> SEKKNYSALFENLQNRSNPEKLQEITTKFFSDNPDVKYNDVLKYITLAMNGVSPEYTNKSREAGEKVKLHLQDILLDVEYQYQGSVM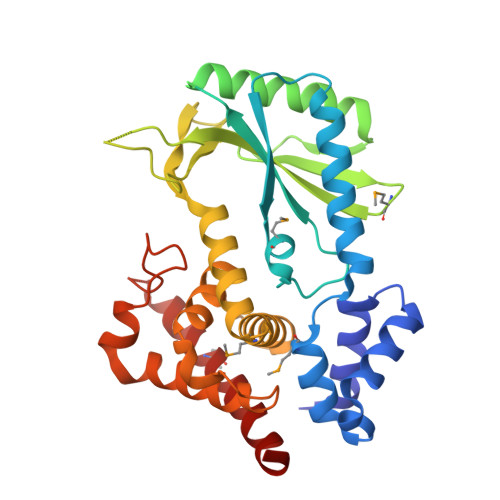TNTHIKGYSDIDLLVISDKFYTLDERNIIENLEVNKFSLSQEKIQKLQQELLGKKYHSATNDLKNNRLLSEQKLSSVYEICDITHPKAIKITNKSMGRDVDIVIANWYDDAQSVINNRQIEYRGIQIYNKRSNTIENRDFPFLSIQRINKRSSETKGRLKKMIRFLKNLKADSDEKIELSSFDINAICYNIEKNKYLHSNKYQLVPILYEQLNELVSNSNKINSLKSVDGHEYIFSRNNIDKKESLKMLLQEVKIIYSNLQSYL> GHMGAASASLAIGGVVIIGGGGHAKVVIESLRACGETVAAIVDADPTRRAVLGVPVVGDDLALPMLREQGLSRLFVAIGDNRLRQKLGRKARDHGFSLVNAIHPSAVVSPSVRLGEGVAVMA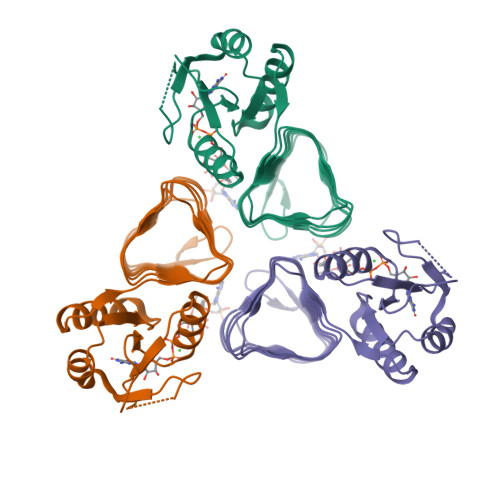GVAINADSWIGDLAIINTGAVVDHDCRLGAACHLGPASALAGGVSVGERAFLGVGARVIPGVTIGADTIVGAGGVVVRDLPDSVLAIGVPAKIKGDRS> MMPVFHTRTIESILEPVAQQISHLVIMHEEGEVDGKAIPDLTAPVAA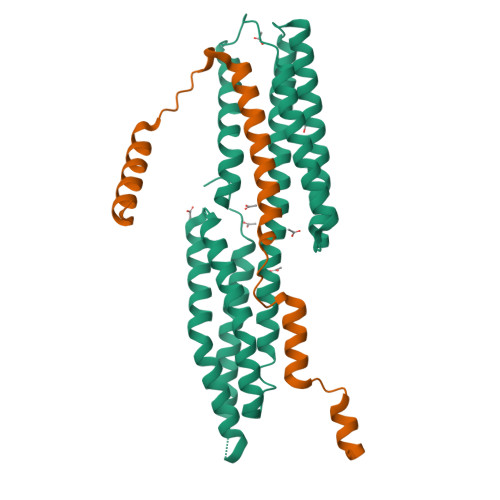VQAAVSNLVRVGKETVQTTEDQILKRDMPPAFIKVENACTKLVQAAQMLQSDPYSVPARDYLIDGSRGILSGTSDLLLTFDEAEVRKIIRVCKGILEYLTVAEVVETMEDLVTYTKNLGPGMTKMAKMIDERQQELTHQEHRVMLVNSMNTVKELLPVLISAMKIFVTTKNSKNQGIEEALKNRNFTVEKMSAEINEIIRVLQLTS;> GPLGSELAYALNNFDKQIIVDPLSFSEERFRPSLEERLESIISGAALMADSSCTRDDRRERIVAECNAVRQALQDLLSEYMGNAGRKERSDALNSAIDKMTKKTRDLRRQL> DRHHHHHHKLVPLAPADRAPAVGQFWHVTDLHLDPTYHITDDRTKVCASSKGANASNPGPFGDVLCDSPYQLILSAFDFIKNSGQEASFMIWTGDSPPHVPVPELSTGTVIKVITNMTMTVQNLFPNLQVFPALGNHDYWPQDQLPIVTSKVYSAVADLWKPWLGEEAISTLKKGGFYSQKVASNPGLRIISLNTNLYYGPNIMTLNKTDPANQFEWLENTLNSSLWNKEKVYIIAHVPVGYLPYATDTPAIRQYYNEKLLDIFRRYSSVIAGQFYGHTHRDSLMVLSDKNGNPLNSVFVAPAVTPVKGVLQKETNNPGVRLFQYKPGDYTLLDMVQYYLNLTEANLKGESNWTLEYVLTQAYSVADLQPKSLYALVQQ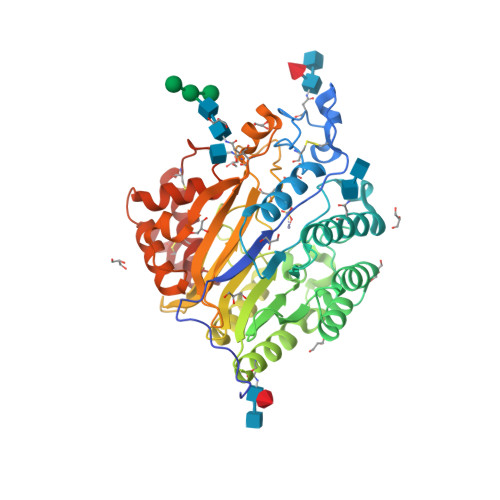FATKDSKQFLKYYHYYFVSYDSSATCDQHCKTLQVCAIMNLDSMSYDDCLKQHL3-(5-chloranyl-1,3-benzothiazol-2-yl)propanoic 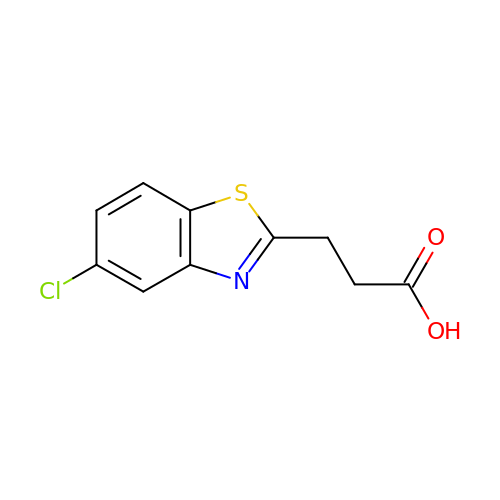acid | C10 H8 Cl N O2 S | UMBLVHSXXWQLDL-UHFFFAOYSA-N>MTKNYYDRSVSPVEYAYFDQSQNMRAINWNKIVDEKDLEVWNRVTQNFWLPENIPVSNDLPSWNELDDDWQQLITRTFTGLTLLDTVQSSIGDVAQIKNSLTEQEQVIYANFAFMVGVHARSYGTIFSTLCTSEQIEEAHEWVVDNEALQARPKALIPFYTADDPLKSKIAAALMPGFLLYGGFYLPFYLSARGKLPNTSDIIRLILRDKVIHNFYSGYKYQLKVAKLSPEKQAEMKQFVFDLLDKMIGLEKTYLHQLYDGFGLADEAIRFSLYNAGKFLQNLGY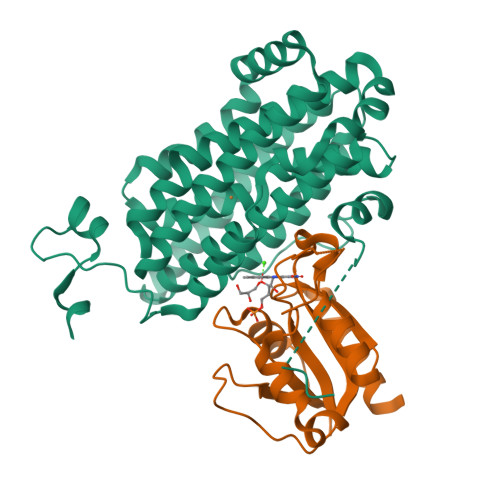ESPFTKEETRIAPEVFAQLSARADENHDFFSGSGSSYIIGTSEETLDEDWDF[4x];>MKELIVYFSTQSNNTHRFVQKLDAESIRIPIDEEERIKVDEDYVLIVPTYSGGKVTDAGQVDAHGAVPKQVIHFLNDPDNRKHCLGVISSGNTNFGDSFAIAGPVISYKLKVPLLYQFELIGTKEDVEEVNRIISETFNADQ[4x]>QKPAACRCSRQDPKNRVNCGFPGITSDQCFTSGCCFDSQVPGVPWCFKPLPAQESEECVMQVSARKNCGYPGISPEDCAARNCCFSDT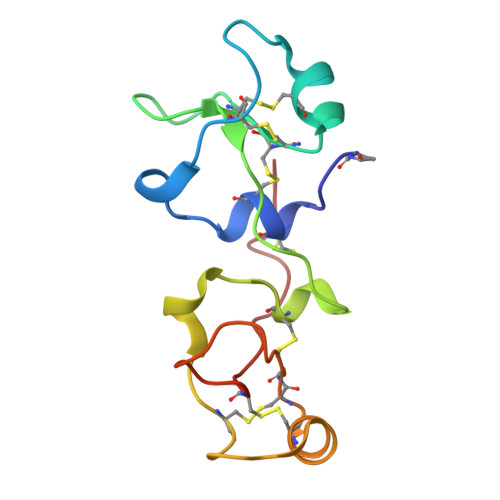IPEVPWCFFPMSVEDCHY[2x]>[2x]SNAQECSLQSCTQHQPYVVDDPCPIHFYSKWYIRVGARKSAPLIELCVDEAGSKSPIQYIDIGNYTVSCLPFTINCQEPKLGSLVVRCSFYEDFLEYHDVRVVLDFI

SARS-CoV-2 ORF8 is a 121-amino acid (aa) protein consisting of an N-terminal signal sequence followed by a predicted Ig-like fold. The accessory protein ORF8 is one of the most rapidly evolving betacoronavirus proteins (1–7). ORF8 disrupts IFN-I signaling when exogenously overexpressed in cells. It has been shown that ORF8 of SARS-CoV-2, but not ORF8 or ORF8a/ORF8b of SARS-CoV, down-regulates MHC-I in cells. The structure of the SARS-CoV-2 ORF8 protein reveals two novel intermolecular interfaces layered onto an ORF7 fold.

The structure of SARS-CoV-2 ORF8 was determined by X-ray crystallography at a resolution of 2.04 Å. ORF8 crystallized as a covalent dimer with three sets of intramolecular disulfide bonds per monomer and a single intermolecular disulfide bond formed by Cys20 of each monomer. The core of each ORF8 monomer consists of two antiparallel β-sheets. Punctuated between what would be β3 and β5 of ORF7a is an ORF8-specific region of ∼35 aa from residues 46 to 83 that are structurally distinct from ORF7a and other Ig-like folds. These residues are responsible for a third, ORF8-specific, disulfide. The dimeric interface amounts to ∼1,320 Å2 in buried surface area. Val117 forms a hydrophobic interaction with its symmetry-related counterpart. This central hydrophobic region is flanked by salt bridges between Arg115 and Asp119. The ends of the interface are stabilized by a “clamp” loop which makes main-chain hydrogen bonding interactions between Phe120 of one subunit and Ala51 and Arg52 of the other. The structure reported here is of the Leu84 form.> MASYPKLTGTVIGTQGSWNNIGNTIHKAFDGDLNTFFDGPTANGCWLGLDFGEGVRNVITQIKFCPRSGYEQRMIGGIFQGANKEDFS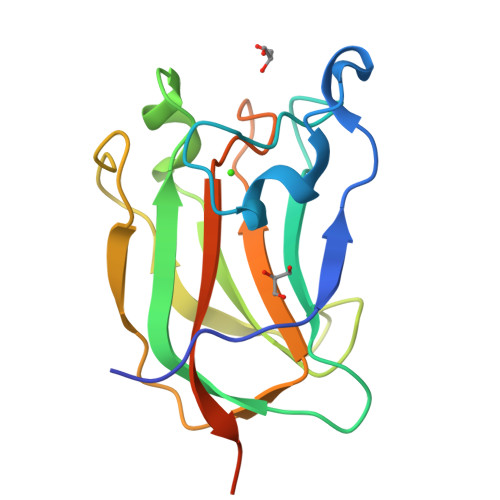DAVTLFTITSLPGSGTLTSVDVDNPTGFRYVRYLSPDGSNGNIAELQFFGTPAGEENDDLEHHHHHH> MMKAKVIDAVSFSYILRTVGDFLSEANFIVTKEGIRVSGIDPSRVVFLDIFLPSSYFEGFEVSQEKEIIGFKLEDVNDILKRVLKDDTLILSSNESKLTLTFDGEFTRSFELPLIQVESTQPPSVNLEFPFKAQLLTITFADIIDELSDLGEVLNIHSKENKL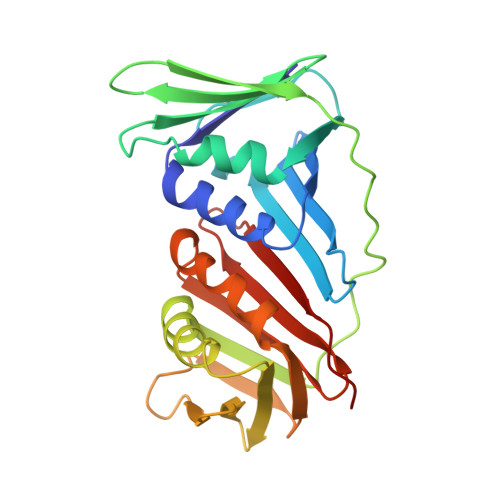YFEVIGDLSTAKVELSTDNGTLLEASGADVSSSYGMEYVANTTKMRRASDSMELYFGSQIPLKLRFKLPQEGYGDFYIAPRAD> GDVLKDRPQEADGIDSVIVVDNVPQVGPDRLEKLKNVIHKIFSKFGKITNDFYPEEDGKTKGYIFLEYASPAHAVDAVKNADGYKLDKQHTFRVNLF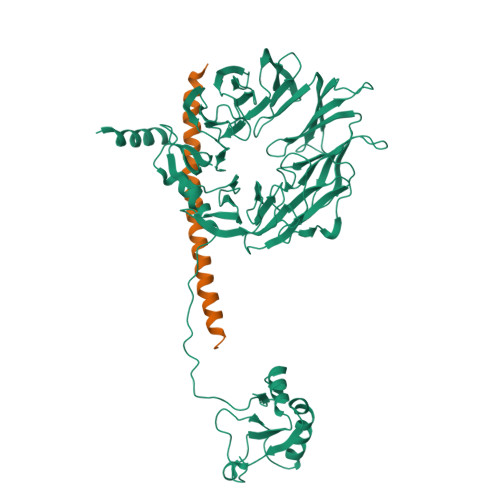TDFDKYMTISDEWDIPEKQPFKDLGNLRYWLEEAECRDQYSVIFESGDRTSIFWNDVKDPVSIEERARWTETYVRWSPKGTYLATFHQRGIALWGGEKFKQIQRFSHQGVQLIDFSPCERYLVTFSPLMDTQDDPQAIIIWDILTGHKKRGFHCESSAHWPIFKWSHDGKFFARMTLDTLSIYETPSMGLLDKKSLKISGIKDFSWSPGGNIIAFWVPEDKDIPARVTLMQLPSRQEIRVRNLFNVVDCKLHWQKNGDYLCVKVDRTPKGTQGVVTNFEIFRMREKQVPVDVVEMKETIIAFAWEPNGSKFAVLHGEAPRISVSFYHVKSNGKIELSKMFDKQQANTIFWSPQGQFVVLAGLRSMNGALAFVDTSDCTVMNIAEHYMASDVEWDPTGRYVVTSVSWWSHKVDNAYWLWTFQGRLLQKNNKDRFCQLLWRPRPPTLLSQEQIKQIKKDLKKYSKIFEQKDRLSQSKASKE tert-butyl 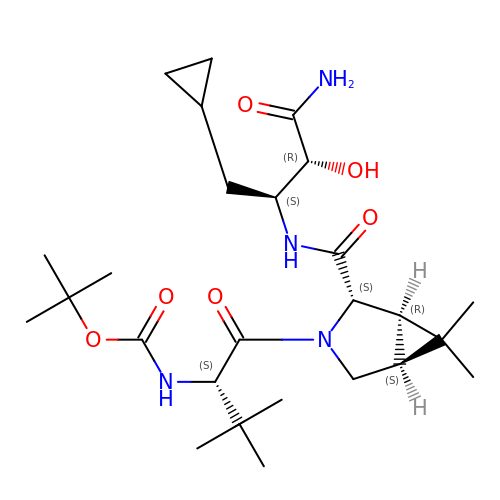{(2S)-1-[(1R,2S,5S)-2-{[(2S,3R)-4-amino-1-cyclopropyl-3-hydroxy-4-oxobutan-2-yl]carbamoyl}-6,6-dimethyl-3-azabicyclo[3.1.0]hex-3-yl]-3,3-dimethyl-1-oxobutan-2-yl}carbamate | C26 H44 N4 O6 | LJEXABSCSDSMLF-XREYTECCSA-N>[2x]MDYKDDDDKENLYFQGDVVDPDIFNRDPRDHYDLLQRLGGGTYGEVFKARDKVSGDLVALKMVKMEPDDDVSTLQKEILILKTCRH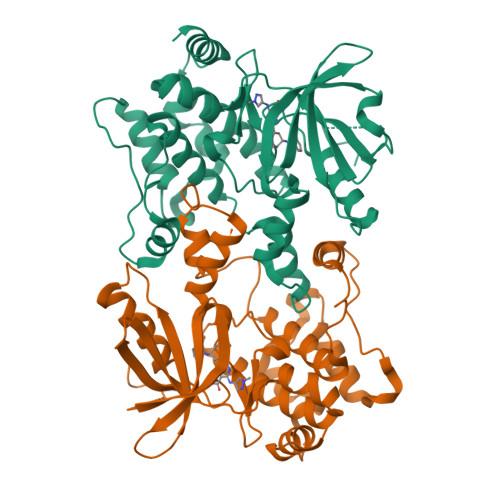ANIVAYHGSYLWLQKLWICMEFCGAGSLQDIYQVTGSLSELQISYVCREVLQGLAYLHSQKKIHRDIKGANILINDAGEVRLADFGISAQIGATLARRLSFIGTPYWMAPEVAAVALKGGYNELCDIWSLGITAIELAELQPPLFDVHPLRVLFLMTKSGYQPPRLKEKGKWSAAFHNFIKVTLTASPAARPSATKMLSHQLVSQPGLNRGLILDLLDKLKNPG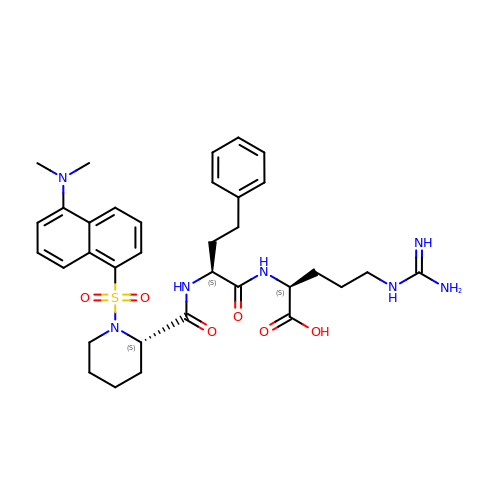(2~{S})-5-carbamimidamido-2-[[(2~{S})-2-[[(2~{S})-1-[5-(dimethylamino)naphthalen-1-yl]sulfonylpiperidin-2-yl]carbonylamino]-4-phenyl-butanoyl]amino]pentanoic acid | C34 H45 N7 O6 S | MKNCAFDCRIGOAN-YCVJPRETSA-N>SNAMIIRPEQHWFLRLFDWHGSVLSKIIFRLLLNVLMSIIAIISYQWYEQLGIHLTVAPFSLLGIAIAIFLGFRNSASYSRFVEARNLWGTVLIAERTLVRQLRNILPAEHDAHRRIVSYLVAFSWSLKHQLRKTDPTADLRRLLPEERVTEILASSMPTNRILLLAGNEIGQLREAGKLSDITYGLMDNKLDELAHVLGGCERLATTPVPFAYTLILQRTVYLFCTLLPFALVGDLHYMT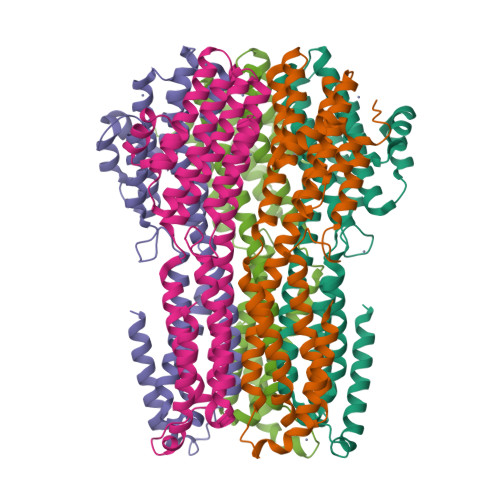PFVSVFISYTFLSWDSLAEELEDPFGTAANDLPLNAMCNTIERNLLDMTGQHPLPE[5x]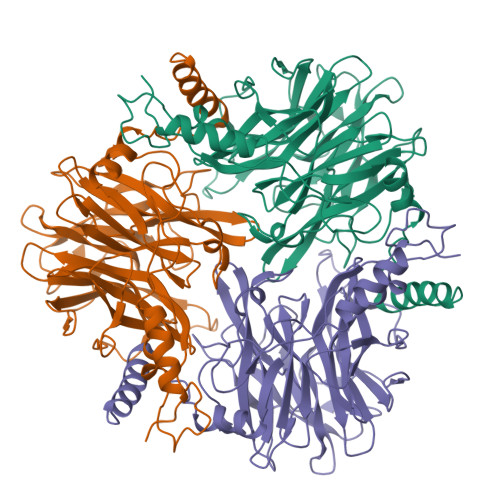> MIHEKYTEMRNEQEALLSRKNTKTSFYNGIYDRYEHPVLTREHIPLHWRYDLNKETNPFFQERLGINAVFNAGAIKLNDRYCLVARVEGNDRKSFFAVAESDKGTEGFRFRQYPVCLPALTDDETNVYDMRLTQHEDGWIYGVFCVEKSAGTADLSEAVASAGIARTKDLTNWERLPDLVTLRSPQQRNVTLLPEFVDGKYAFYTRPMDGFIETGSGGGIGFGLADDITHAVIDEERMTSIRRYHTITESKNGAGATPIKTERGWLNIAHGVRNTAAGLRYVIYCFVTDLSEPWKVIAEPGGYLIAPFKDERVGDVSNVVFTNGAIVDDNGDVYIYYASSDTRLHVAVSSIDKLLDYAFNTPADALRTAECVKQRCDLIKRNIELL> TTSEKVFPKINVLIVEDNVINQAILGSFLRKHKISYKLAKNGQEAVNIWKEGGLHLIFMDLQLPVLSGIEAAKQIRDFEKQNGIGIQKSLNNSHSNLEKGTSKRFSQAPVIIVALTA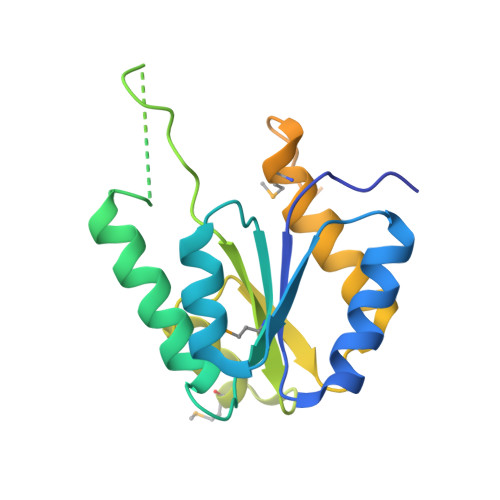SNSQMDKRKALLSGCNDYLTKPVNLHALSKKITEWGCMQALIDFDSWKQGESRMTDSVLVKSPQKPIAPSNPHSFKQATSMTPTHSPVRKNSNLSPTQIEL>MVFESELLLQRRLATTALKQPKELGYYSTNVGGELKVMDESNLSYYYL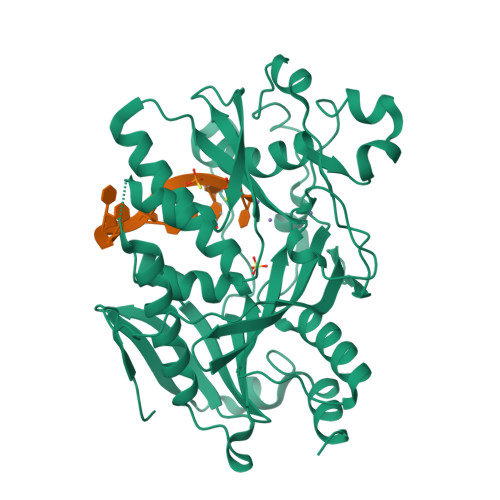PDADIEKHIDLSAGARKFQDEQAEAEDDTGSLHGLLQTLMEYERRKSKKVNADIIAFRGQVKRLIHCAFGGHATDVDMYVMSFDGQLFIRAARKKLEFPTSPRESWAYLAYYSGYKFERMALLDRPVAETPREVLESRGKQVVRNGPQYKTVVRTGVGEHKLVLGAEVDGIFDFREPTGDNLKHYVELKVAKKVQTLKDATNFEQKLFSVWLQCFLVGINRVIIGFRDEKFVLKSVEEFSTSEIPLLLKSTGLRNACVDAIKWYGALTKWLCELPRGPEDDFKLYRLSCSRGALHLRQLHDEDLANGDDIIPGWFREWRRSLSKSHGS[2x]>[4x]GQEQSILDKLVVLPSGEYNHSEAAAMKQRLEKIPTSILDALYSKGVK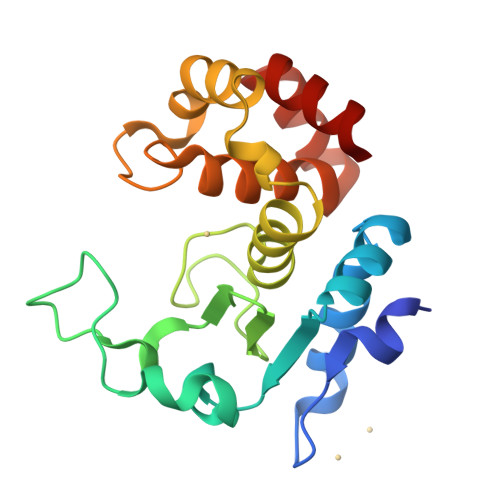IKLTQGAITNEPELAYLKGVVPRGWEGTGLTWDDVPGVSERVVAVRIGYSEKGKGHNSLNLEIHETLHAVDRLVLNEVSGTDEFINIFNKEASVKYKGDGYVSAYPTEYFAEAASLYLYSDATRSDLKDSMPLTYEFMAKLFAN N-(tert-butoxycarbonyl)-L-alanyl-N-[(1R)-1-(dihydroxyboranyl)-2-methylpropyl]-L-prolinamide | C17 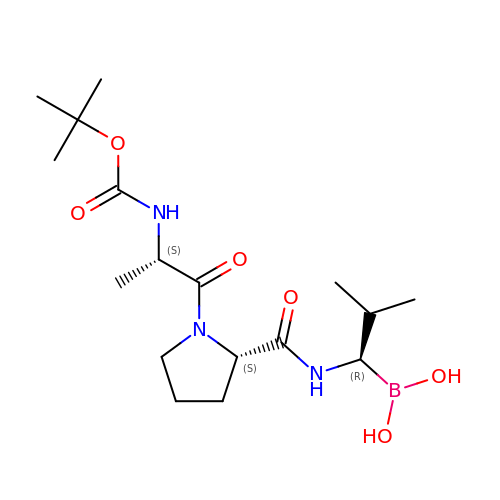H32 B N3 O6 | VWVBZPYREZAAER-AVGNSLFASA-N>[2x]GMIGDGIENSPLLTDLAFPYRLLGAGKESRECLFLLHGSGVDETTLVPLARRIAPTATLVAARGRIPQEDGFRWFERIDPTRFEQKSILAETAAFA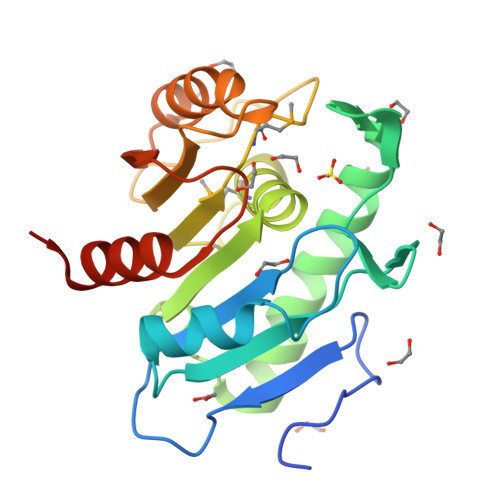AFTNEAAKRHGLNLDHATFLGYSNGANLVSSLMLLHPGIVRLAALLRPMPVLDHVPATDLAGIRTLIIAGAADETYGPFVPALVTLLSRHGAEVDARIIPSGHDIGDPDAAIVRQWLAGPIAIAQAD>SNAMEIIFYHPTFNAAWWVNALEKALPHARVREWKVGDNNPADYALVWQPPVEMLAGRRLKAVFVLGAGVDAILSKLNAHPEMLDASIPLFRLEDTGMGLQMQEYAVSQVLHWFRRFDDYQALKNQALWKPLPEYTREEFSVGIMGAGVLGAKVAESLQAWGFPLRCWSRSRKSWPGVESYVGREELRAFLNQTRVLINLLPNTAQTVGIINSELLDQLPDGAYVLNLARGVHVQEADLLAALDSGKLKGAMLDVFSQEPLPQESPLWRHPRVAMTPHIAAVTRPAEAI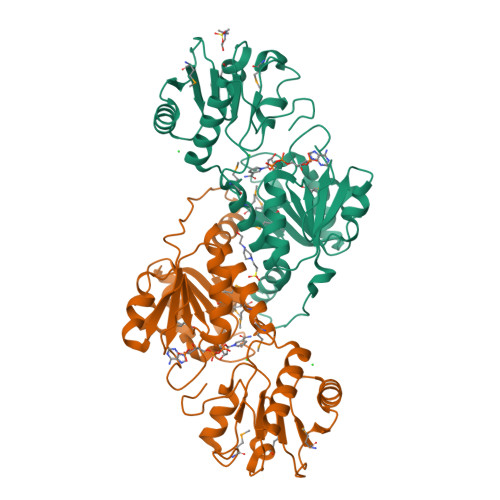DYISRTITQLEKGEPVTGQVDRARGY[4x]> SSTHVNAQKEIENRYKEVKIRIESTVAGSLRSMKSVLEHLRAKMQRMEEAIKTQKELCSAPCTVNCRVPVVSGMHCEDIYRNGGRTSEAYYIQPDLFSEPYKVFCDMESHGGGWTVVQNRVDG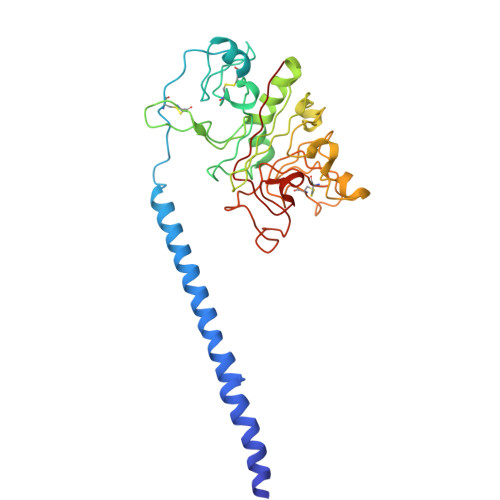SSNFARDWNTYKAEFGNIAFGNGKSICNIPGEYWLGTKTVHQLTKQHTQQVLFDMSDWEGSSVYAQYASFRPENEAQGYRLWVEDYSGNAGNALLEGATQLMGDNRTMTIHNGMQFSTFDRDNDNWNPGDPTKHCSREDAGGWWYNRCHAANPNGRYYWGGIYTKEQADYGTDDGVVWMNWKGSWYSMRQMAMKLRPKWP> MRINHNIAALNTLNRLSSNNSASQKNMEKLSSGLRINRAGDDAAGLAISEKMRGQIRGLEMASK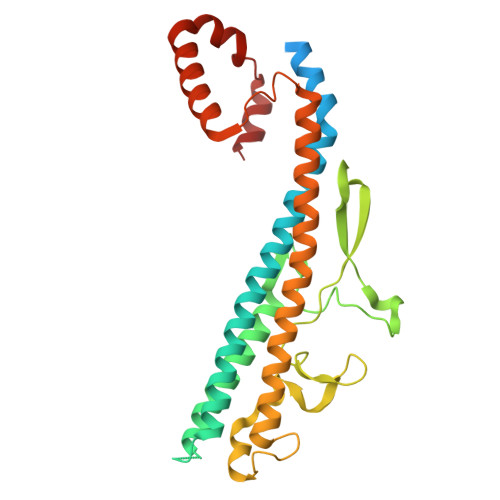NSQDGISLIQTAEGALTETHAILQRVRELVVQAGNTGTQDKATDLQSIQDEISALTDEIDGISNRTEFNGKKLLDGTYKVDTATPANQKNLVFQIGANATQQISVNIEDMGADALGIKEADGSIAALHSVNDLDVTKFADNAADTADIGFDAQLKVVDEAINQVSSQRAKLGAVQNRLEHTINNLSASGENLTAAESRIRDVDMAKEMSEFTKNNILSQASQAMLAQANQQPQNVLQLLR> GASEPMRPGVIRFGLTPVFLSND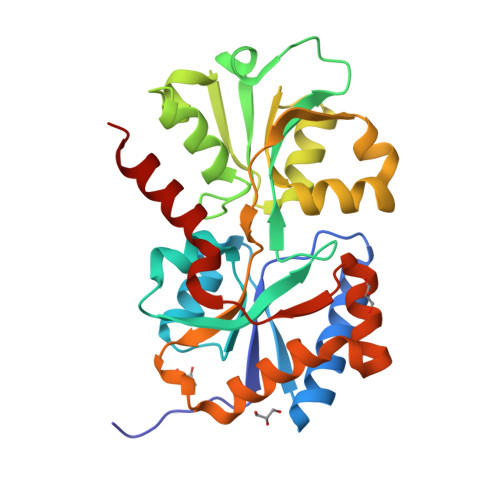LEVLDELQAYLTQAVGQEVQLITQRTYQEVTALLVSGNLEAAWICGYPFMKFRDELDLVATPLWRGKPVYQSYLIVGRDRDIAGFEDCQGDIHAFSDPDSNSGYLVTKTYLAERGVSEEGFFRKSFFTYGHRNVIRAVASGLADSGSVDGYVWEVMKTTEPELVAKTRVLVKSGWHGFPPVAAAAGQRKSQAVARIRSALLDMNQEVLGRSVLTRLQLDGFVETTAESYDSIAANMERVRRLG>MSRNNDINAEVVSVSPNKLKISVDDLEEFKIAEEKLGVGSYLRVSDNQDVALLAIIDNFSIEVKESQKQKYMIEASPIGLVKNGKFYRGGDSLALPPKKVEPAKLDEIISIYSDSIDINDRFTFSSLSLNTKVSVPVNGNRFFNKHIAIVGSTGSGKSHTVAKILQKAVDEKQEGYKGLNNSHIIIFDIHSEYENAFPNSNVLNVDTLTLPYWLLNGDELEELFLDTEANDHNQRNVFRQAITLNKKIHFQGDPATKEIISFHSPYYFDINEVINYINNRNNERKNKDNEHIWSDEEGNFKFDNENAHRLFKENVTPDGSSAGALNGKLLNFVDRLQSKIFDKRLDFILGEGSKSVTFKETLETLISYGKDKSNITILDVSGVPFEVLSICVSLISRLIFEFGYHSKKIKRKSNENQDIPILIVYEEAHKYAPKSDLSKYRTSKEAIERIAKEGRKYGVTLLLASQRPSEISETIFSQCNTFISMRLTNPDDQNYVKRLLPDTVGDITNLLPSLKEGEALIMGDSISIPSIVKIEKCTIPPSSIDIKYLDEWRKEWVDSEFDKIIEQWSKS[6x];>MDRSAVDTIRGYCYQVDKTIIEIFSLPQMDDSIDIECIEDVDVYNDGHLTAIQCKYYESTDYNHSVISKPIRLMLSHFKDNKEKGANYYLYGHYKSGQEKLTLPLKVDFFKSNFLTYT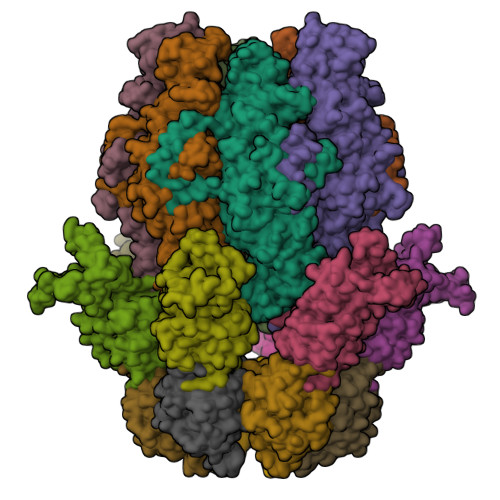EKKIKHEYHIENGLTEEDLQAFLDRLVININAKSFDDQKKETIQIIKNHFQCEDYEAEHYLYSNAFRKTYDISCNKKDRRIKKSDFVESINKSKVLFNIWFYQYEGRKEYLRKLKESFIRRSVNTSPYARFFILEFQDKTDIKTVKDCIYKIQSNWSNLSKRTDRPYSPFLLFHGTSDANLYELKNQLFNEDLIFTDGYPFKGSVFTPKMLIEGFSNKEIHFQFINDIDDFNETLNSINIRKEVYQFYTENCLDIPSQLPQVNIQVKDFADIKEIV[12x]(1~{R},3~{S},5~{Z})-5-[2-[(1~{R},3~{a}~{S},7~{a}~{R})-7~{a}-methyl-1-[(6~{R})-1,1,1-tris(fluoranyl)-10-methyl-2,10-bis(oxidanyl)-2-(trifluoromethyl)undeca-3,8-diyn-6-yl]-2,3,3~{a},5,6,7-hexahydro-1~{H}-inden-4-ylidene]ethylidene]-4-methylidene-cyclohexane-1,3-diol 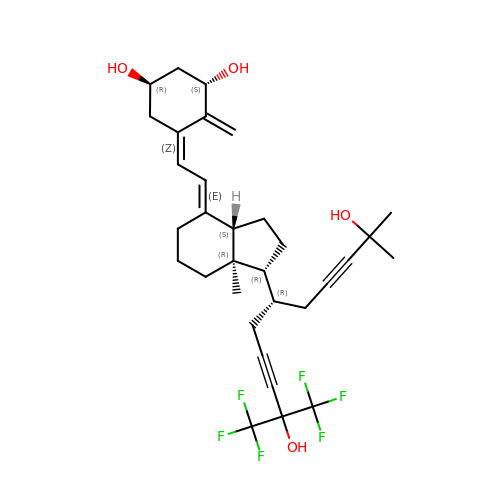| C32 H40 F6 O4 | IOHHJACKQNKBKZ-GEJQTTJQSA-N4-[2-[[(2~{R})-2-phenylpropyl]amino]ethyl]benzene-1,2-diol | 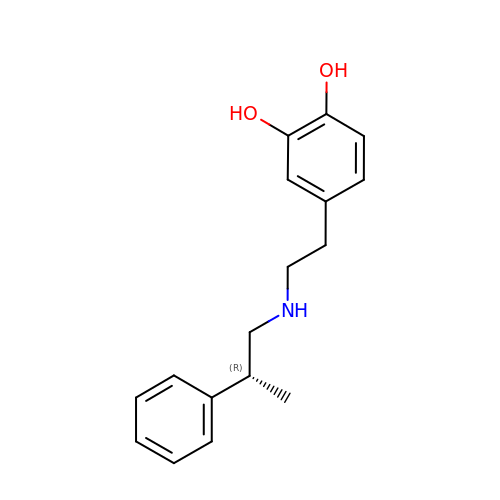C17 H21 N O2 | NXTJHSKVIAFFNX-ZDUSSCGKSA-N>[6x]MSLKRFDLIIRSSTVVTETTTYRADVAIRNGIVSAITEPGSISSDDGPAIDGTGLHLFPGMVD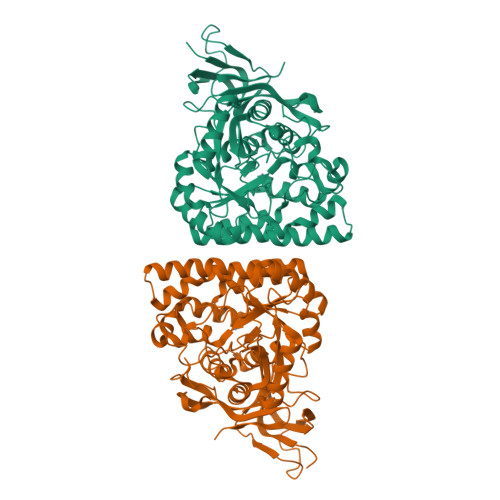VHVHFNEPGRTEWEGFASGSKSLAAGGVTTYFDMPLNSNPPTITREELDKKRQLANEKSLVDYRFWGGLVPGNIDHLQDLHDGGVIGFKAFMSECGTDDFQFSHDETLLKGMKKIAALGSILAVHAESNEMVNALTTIAIEEQRLTVKDYSEARPIVSELEAVERILRFAQLTCCPIHICHVSSRKVLKRIKQAKGEGVNVSVETCPHYLLFSLDEFAEIGYLAKCAPPLRERQEVEDLWDGLMAGEIDLISSDHSPSLPQMKTGKTIFEVWGGIAGCQNTLAVMLTEGYHKRKMPLTQIVQLLSTEPAKRFGLYPQKGTIQVGAEASFTLIDLNESYTLNASDLYYRHPISPYVGQRFRGKVKHTICQGKHVYQDHEGHHHHHH>MLCEIECRALSTAHTRLIHDFEPRDALTYLEGKNIFTEDHSELISKMSTRLERIANFLRIYRRQASELGPLIDFFNYNNQSHLADFLEDYIDFAINEPDLLRPVVIAPQFSRQMLDRKLLLGNVPKQMTCYIREYHVDRVIKKLDEMCDLDSFFLFLHGRAGSGKSVIASQALSKSDQLIGINYDSIVWLKDSGTAPKSTFDLFTDILLMLKSEDDLLNFPSVEHVTSVVLKRMICNALIDRPNTLFVFDDVVQEETIRWAQELRLRCLVTTRDVEISNAASQTCEFIEVTSLEIDECYDFLEAYGMPMPVGEKEEDVLNKTIELSSGNPATLMMFFKSCEPKTFEKMAQLNNKLESRGLVGVECITPYSYKSLAMALQRCVEVLSDEDRSALAFAVVMPPGVDIPVKLWSCVIPVDICSNEEEQ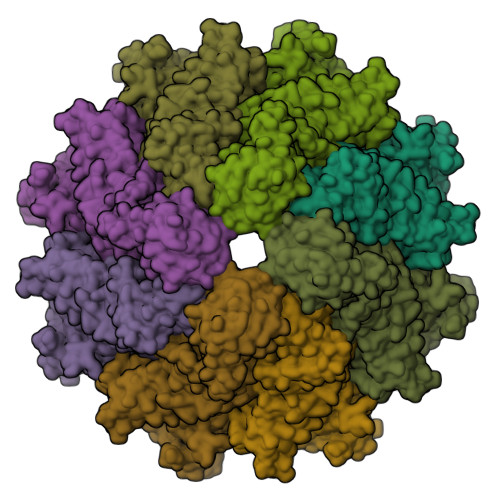LDDEVADRLKRLSKRGALLSGKRMPVLTFKIDHIIHMFLKHVVDAQTIANGISILEQRLLEIGNNNVSVPERHIPSHFQKFRRSSASEMYPKTTEETVIRPEDFPKFMQLHQKFYDSLKNFACC[2x];>PLFNFMGC[2x]> GSGRSDTVPSPRDLQ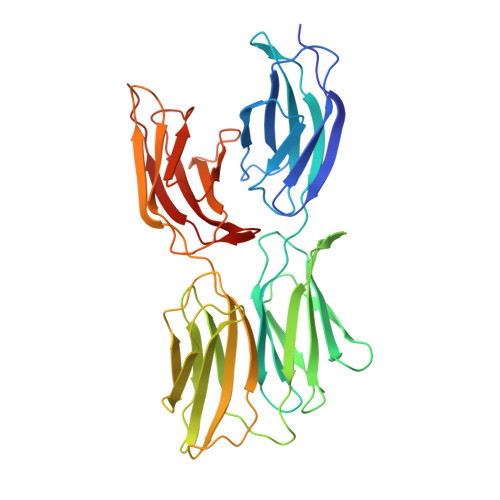FVEVTDVKVTIMWTPPESAVTGYRVDVIPVNLPGEHGQRLPISRNTFAEVTGLSPGVTYYFKVFAVSHGRESKPLTAQQTTKLDAPTNLQFVNETDSTVLVRWTPPRAQITGYRLTVGLTRRGQPRQYNVGPSVSKYPLRNLQPASEYTVSLVAIKGNQESPKATGVFTTLQPGSSIPPYNTEVTETTIVITWTPAPRIGFKLGVRPSQGGEAPREVTSDSGSIVVSGLTPGVEYVYTIQVLRDGQERDAPIVNKVVTPLSPPTNLHLEANPDTGVLTVSWERSTTPDITGYRITTTPTNGQQGNSLEEVVHADQSSCTFDNLSPGLEYNVSVYTVKDDKESVPISDTIIPAVP>[2x]MVKKKEPAEGWPVVSGDYIVGDPESPVAAVTLASHIEDIPIDAGAAIAGPCKTENLGIEKVIANIISNPNIRFLVLCGSEVQGHIVGQSMKALHKNGVDDKRKIIGAKGAIPYIENLPEEALERFQKQVEIVDLIDVEDADQIKEKVKECIEKDPGAFEEEEVILRL;> GSHMVKKKEPAEGWPVVSGDYIVGDPESPVAAVTL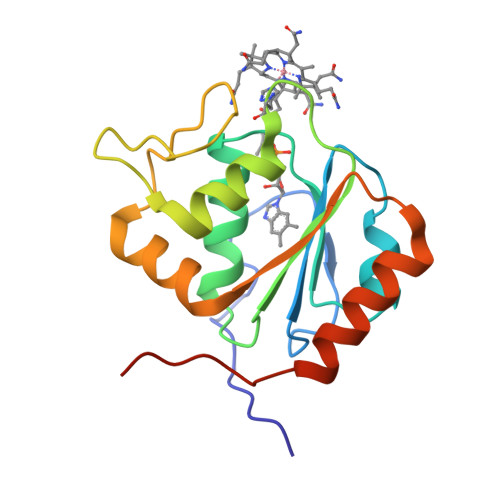ASHIEDIPIDAGAAIAGPCKTENLGIEKVIANIISNPNIRFLVLCGSEVQGHIVGQSMKALHKNGVDDKRKIIGAKGAIPYIENLPEEALERFQKQVEIVDLIDVEDADQIKEKVKECIEKDPGAFEEEEVILRL> METAMSKGVITITDAEFESEVLKAEQPVLVYFWASWCGPCQLMSPLINLAANTYSDRLKV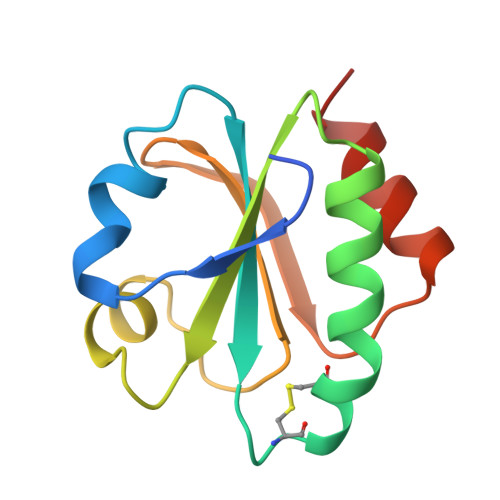VKLEIDPNPTTVKKYKVEGVPALRLVKGEQILDSTEGVISKDKLLSFLDTHLNNN N-[(4-hydroxyphenyl)methyl]adenosine | C17 H19 N5 O5 | 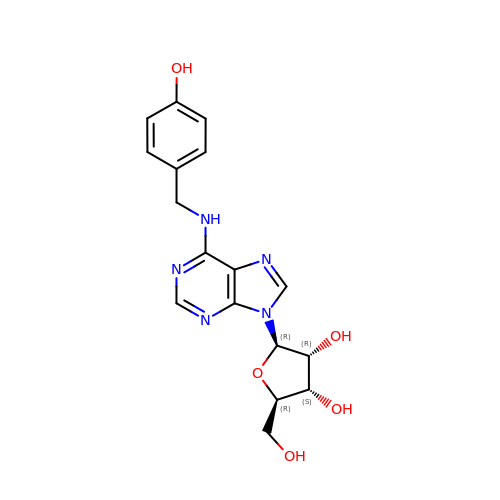UGVIXKXYLBAZND-LSCFUAHRSA-N>[2x]GSTGGVQTVTLIPGDGIGPEISAAVMKIFDAAKAPIQWEERNVTAIQGPGGKWMIPSEAKESMDKNKMGLKGPLKTPIAAGHPSMNLLLRKTFDLYANVRPCVSIEGYKTPYTDVNIVTIRENTEGEYSGIEHVIVDGVVQSIKLITEGASKRIAEFAFEYARNNHRSNVTAVHKANIMRMSDGLFLQKCREVAESCKDIKFNEMYLDTVCLNMVQDPSQFDVLVMPNLYGDILSDLCAGLIGGLGVTPSGNIGANGVAIFESVHGTAPDIAGKDMANPTALLLSAVMMLRHMGLFDHAARIEAACFATIKDGKSLTKDLGGNAKCSDFTEEICRRVKDLD;>[2x]ASRSQAEDVRVEGSFPVTMLPGDGVGPELMHAVKEVFKAAAVPVEFQEHHLSEVQNMASEEKLEQVLSSMKENKVAIIGKIHTPMEYKGELASYDMRLRRKLDLFANVVHVKSLPGYMTRHNNLDLVIIREQTEGEYSSLEHESARGVIECLKIVTRAKSQRIAKFAFDYATKKGRGKVTAVHKANIMKLGDGLFLQCCEEVAELYPKIKFETMIIDNCCMQLVQNPYQFDVLVMPNLYGNIIDNLAAGLVGGAGVVPGESYSAEYAVFETGARHPFAQAVGRNIANPTAMLLSASNMLRHLNLEYHSSMIADAVKKVIKVGKVRTSDMGGYATCHDFTEEICRRVKDLDENLYFQ

Human NAD-IDH is a key enzyme in the TCA cycle, which catalyzes the oxidative decarboxylation of ICT into α-KG. The α and β subunits form a heterodimer (αβ), and the α and γ subunits form another heterodimer (αγ), which are assembled into a heterotetramer (α2βγ) and further into a heterooctamer (the heterotetramer and heterooctamer are also called holoenzyme). Our previous biochemical studies demonstrated that the αγ heterodimer alone exhibits a high enzymatic activity and kinetic properties comparable with those of the holoenzyme and can be activated by CIT and ADP but inhibited by NADH; on the other hand, the αβ heterodimer alone exhibits a low activity and cannot be activated by the activators but can be inhibited by NADH. Our structural comparisons show that the αβ heterodimer has a similar yet more compact overall structure compared with the αγ heterodimer and contains a pseudo-allosteric site that exhibits substantial conformational differences from the allosteric site in the αγ heterodimer.

Crystals of the αβ heterodimer with the α subunit bound with a Ca2+ at the active site (αCaβ) grew at condition II and belong to space group I4, and the structure was determined at 3.0 Å resolution with each asymmetric unit containing two αCaβ molecules, which form a dimer of heterodimers via the clasp domains. In this structure, there is evident electron density at the active site, which is interpreted as a Ca2+ due to the presence of 0.2 m Ca2+ in the crystallization solution and a reasonable B factor after structure refinement. We also obtained crystals of the αCaβ heterodimer at condition II in the presence of CIT or/and ADP (both 50 mm); however, in these structures, there is only a Ca2+ bound at the active site and no CIT or ADP bound in either the α or β subunit. Structural analysis shows that in the αCaβ structure, the N-terminal region of helix α7 in both the α and β subunits assumes the active α-helical conformation, and the key residues Tyr-126A and Lys-142A at the active site and Tyr-137B and Lys-153B at the pseudo-allosteric site (equivalent to Tyr-135G and Lys-151G at the allosteric site) also assume active conformations similar to those in the αMgγMg+CIT+ADP heterodimer. In other words, the αCaβ structure exhibits an active overall conformation. In the αCaβ structure, the longer side chain of Gln-132B pushes the side chain of Tyr-137B away to adopt the active conformation, which is stabilized by a hydrogen bond with the side chain of Lys-173A. This hydrogen-bonding interaction also induces the β5B-β6B loop to assume the active conformation, which further triggers the conformational changes of the structure elements at the heterodimer interface and the active site, including the N-terminal region of helix α7 in both the α and β subunits and the β5A-β6A loop at the active site.N-{5-[(7-bromonaphthalen-1-yl)methyl]-1,3-thiazol-2-yl}-2-[(4,6-dimethylpyrimidin-2-yl)sulfanyl]acetamide | C22 H19 Br N4 O S2 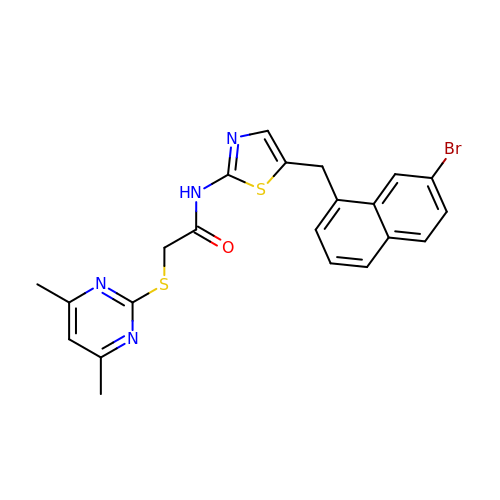| YKVBPTQPNLFGIG-UHFFFAOYSA-N7-CHLOROTETRACYCLINE | C22 H23 Cl N2 O8 | 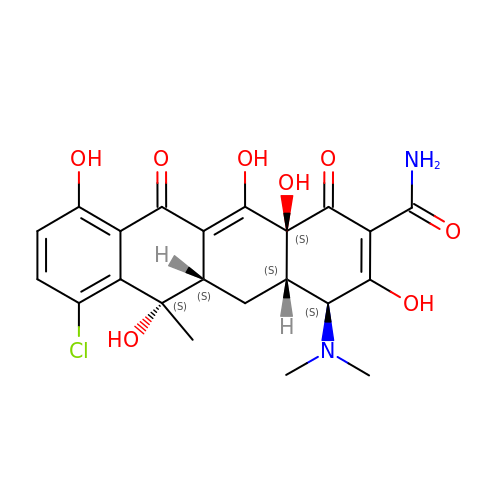CYDMQBQPVICBEU-XRNKAMNCSA-N5-(4-fluorophenyl)-4-[4-fluoro-3-(trifluoromethyl)phenyl]-1H-pyrazole | C16 H9 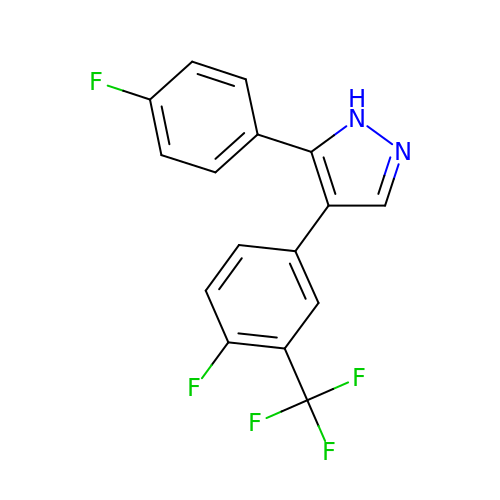F5 N2 | MQERCRUBCCKCNG-UHFFFAOYSA-N>[4x]MIALSANAFETTTPPEPPQFPAEGKINYVARDTILEFKALPSYSEPDWITEKFEKAGKLPPLKERLPEEPLVYKTGNMPDGVGVYGDTMRHVVGGRPEGWNYIAGQSQGWGGIDIALSECLTRTAPLFQVDAKDTEPLPNLAKSWEWSEDGHTLTMHLVKGAKWSDGEAFNADDVMFYWEDAVVDPNVSPLGGGASPEAFGEGTTLKKIDDYTVEWTFKAAFPKQYLYTMAYPSFCPGPSHILKPQHPKYSKNTYNQFKNAFPPEYMNMPVMGAWVPVSYRPDDLIVLRRNPYYWKVDEKGQQLPYLNEVHYKLSTWADRDVQAVAGSGDFSNLEQPENFVASLKRAADPN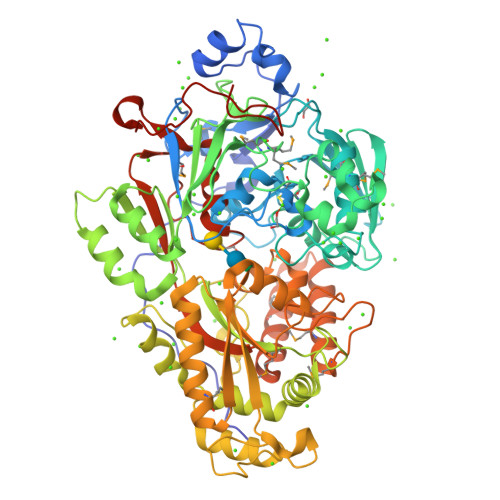APARLAFGPRLIGYNLQMNFSANGWGNPDERGQAIRELNRNEVFRQAVTSALDRKAIGDSLVKGPFTAIYPGGISSGTSFYDRASTVYYPFNLEGAKAALASIGLKDTDGDGFLNFPKETLGGRNVEITLLVNNGYATDKSLAEGLVGQMAKLGLRVVIHSLDSNQRDAAHYGGQFDWLVRRNSTELSSVVQNTEQLAPVGPRTSWNHRSPEGKELDLMPFEKEMADIVRKFISSQDNAERADLMKQYQKVYTQNLYTIGLTEYPGALIVNKRFSNVPQGTPIFMFNWAEDAIIRERLWVAADKQGKYELFPQQLPGKPGEGGPINHHHHHH> YTDESCTFKISLRNFRSILSWELKNHSIVPTHYTLLYTIMSKPEDLKVVKNCANTTRSFCDLTDEWRSTHEAYVTVLEGFSGNTTLFSCSHNFWLAIDMSFEPPEFEIVGFTNHINVMVKFPSIVEEELQFDLSLVIEEQSEGIVKKHKPEIKGNMSGNFTYIID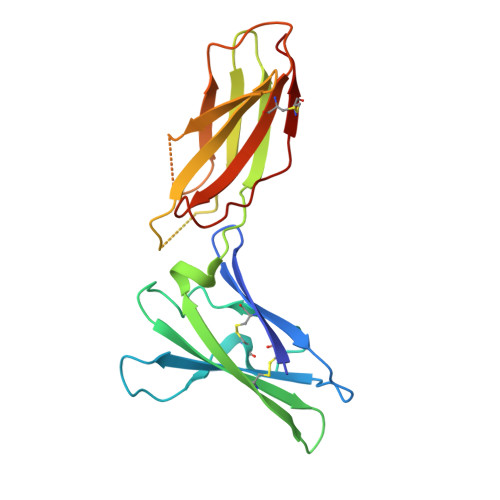KLIPNTNYCVSVYLEHSDEQAVIKSPLKCTLLPP Pseudomonas species and other aerobic bacteria have a biotin-independent malonate decarboxylase that is crucial for their utilization of malonate as the sole carbon and energy source. MdcA, MdcC, MdcD, and MdcE form the 140 kD MDC holoenzyme, with 1:1:1:1 stoichiometry among the four subunits. The malonyl-ACP is decarboxylated in the second step of the reaction to regenerate acetyl-ACP, which is catalyzed by MdcD (30 kD) and MdcE (28 kD).

We next determined the crystal structure at 2.2 Å resolution of the MDC hetero-tetramer, with the MdcA, MdcD, and MdcE subunits from P. aeruginosa and the MdcC subunit from P. fluorescens. The hybrid hetero-tetramer with the P. fluorescens MdcC, which has 76% identity with P. aeruginosa MdcC, produced much better crystals. MdcC did not carry the prosthetic group, as we were not able to express the modifying enzymes in E. coli. A malonate molecule from the crystallization solution is bound in the MdcA active site (see below), so this structure is actually the complex with malonate. The current atomic model has good agreement with the crystallographic data and the expected bond lengths, bond angles and other geometric parameters. The four copies of the hetero-tetramers in the asymmetric unit have similar conformation, with overall rms distances of 0.2–0.4 Å between any pair of their equivalent Cα atoms. The structure therefore indicates that MdcC is an important bridging subunit, mediating the formation of the hetero-tetramer, while the contact between MdcA and MdcD–MdcE (400 Å2) is likely too small to form a stable sub-complex. The active site of MdcA is located at the interface between its AN and AC domains. One of the carboxylates (C1) of malonate has bidentate ion-pair interactions with Arg341, and its two oxygens are also hydrogen-bonded to the side chains of Asn292 and Gln345, respectively. The methylene group (C2) of malonate is situated above the phenyl ring of Phe312.

>[4x]MTTPISPPPQWSRRRQEKQRRLERVRGLADGAVLPREGLVAALEALIAPGDRVVLEGNNQKQADFLSRSLARVDPGKLHDLHMIMPSVGRPEHLDLFELGIARKLDFSFSGPQSLRIGQLLEDGLLEIGAIHTYIELYARLVVDLIPNVALVAGFVADREGNVYTGPSTEDTPALVEPTAFSDGIVIVQVNRIVDDPRDLPRVDIPASWVDFVVEADQPFYIEPLFTRDPRHIKPVHVLMAMMAIRGIYQRHNVQSLNHGIGFNTAAIELILPTYGESLGLKGKICRHWTLNPHPTLIPAIESGWVESVHCFGTELGMEGYIAQRPDVFFTGRDGSLRSNRMFCQLAGQYAVDLFIGATLQVDGDGHSSTVTRGRLAGFGGAPNMGHDPRGRRHSTPAWLDMRGEPEALLERGRKLVVQMVETFQDGGKPTFVERLDALEVARQTGMPLAPVMIYGDDVTHVLTEEGIAYLYKARSLEERQAMIAAVAGISPIGLRHDPRETQRMRREGLIALPEDLGIRRTDASRELLAAKSIAELVEWSGGLYQPPARFRSW;>METLSFEFPAGQPGRGRALVGCVGSGDLEVLLEPGQPGKLSIQVQTSVNGSASRWQHLFERLFDGQTPPALLIDIHDFGATPGVVRLRLEQGFEEIGHD[4x];>MTDVARLLALRSFTELGARQRARALLDAGSFRELLDPFAGVQSPWLERQGIVPQADDGVVVARGLLDGQPAVLAAIEGAFQGGSLGEVSGAKIAGALELAAEDNRNGVPTRALLLLETGGVRLQEANLGLAAIAEIQAAIVDLQRYQPVVAVIAGPVGCFGGMSIAAGLCSYVLVTREARLGLNGPQVIEQEAGIAEYDSRDRPFIWSLTGGEQRFASGLADAYLADDLDEVRTSVLAYFAKGLPARPRCRRAEDYLRRLGDLDTAEQPDAAGVRRLYQGLGQGDAT[4x];>MGSSHHHHHHSQDPNSMSQPFASRGLAWFQALAGSLAPRPGDPASLRVADAELDGYPVRFLAVVPDPDNPFPRARQGEVGLLEGWGLAAAVDEALEADREAPRKRALLAIVDVPSQAYGRREEALGIHQALAGAVDAYARARLAGHPLIGLLVGKAMSGAFLAHGYQANRLIALHDPGVMVHAMGKAAAARITLRSVEELEALAAKVPPMAYDIDSYASLGLLWRTLPVETVEVPSTADLVRVRTCLGEALADILGGPRDLGGRLGAANREASARVRRLLREQW[4x]> PRTARHAPAV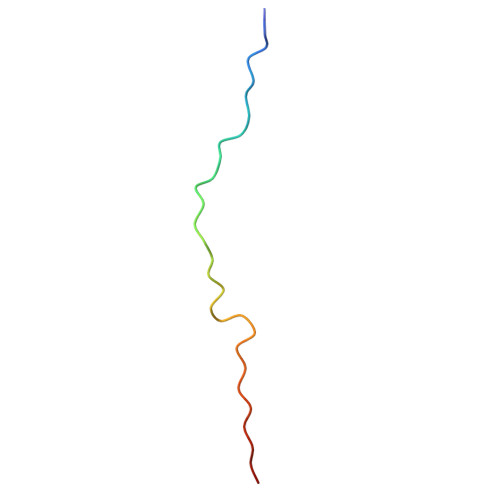RKFSPDLKLLKDVKISVSFTE> METKWLLSKVPDDKSRFEIELEFVQMLSNPWYLNFLAQHKYFEDEAFLQYLEYMEYWREPEYVKFIIYPT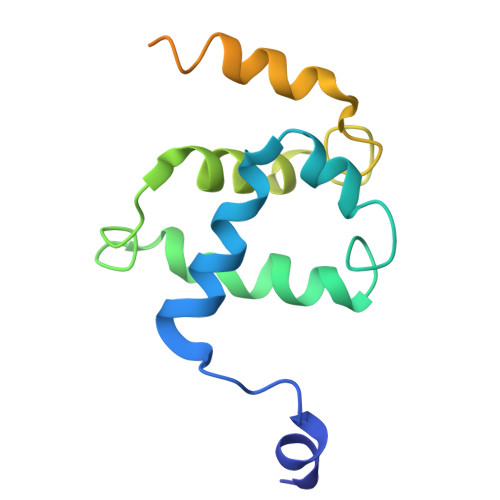CLHMLTLLKNPQFRNDISRADLSKQVNDEIYYEWLGKGLQQYGSADDATLSQPQQEEDEKKVDVKKENE RNA helicase DDX21 plays vital roles in ribosomal RNA biogenesis, transcription, and the regulation of host innate immunity during virus infection. DDX21 is composed of three domains, including the N‐terminal domain, the middle D1 and D2 domain, and the C‐terminal foldase domain. In summary, here we reported multiple sets of crystal structures of RNA helicase DDX21 either in ligand‐free (DDX21‐apo) or in complex with AMP (DDX21‐AMP), ADP (DDX21‐ADP), or a nonhydrolyzable ATP analog (AMPPNP) and a 15‐nucleotide poly(U) ssRNA (DDX21‐AMPPNP‐U15), corresponding to different unwinding states (except for DDX21‐AMP). We elucidated the conformational rearrangements upon the ATP and ssRNA binding during the dsRNA unwinding cycle, and described an RNA unwinding machinery including one wedge helix, one sensor motif V, and the DEVD box.

Therefore, we deleted the linker loop partially (GKKTQ; residue 401‐405) and generated a new construct (named as a del‐loop mutant), which helped us obtain a 1.8 Å resolution crystal structure of DDX21‐ADP and another DDX21‐apo structure with 3.1 Å resolution. Here, we have shown that the DDX21 helicase core adopted an open conformation in its apo‐state, and the success of crystallization either without the linker loop or del‐loop constructs indicated the vast flexibility of the open conformation in solution. When DDX21 was in the apo‐state, the RNA binding pocket was closed tightly. Three motifs in the D1 domain sterically clashed with the modeled ssRNA molecule, including residue Gly295 from motif Ib, residue Asp321 from motif Ic, and more significantly, residues Met347 and Phe349 adjacent to Gln352 which interacted with U4 in the RNA bound structure. A short loop (TGTG, named as “TG loop”) within the motif I had severe steric hindrance with the modeled AMPPNP in DDX21 apo‐structure; thus the ATP‐binding pocket was in the closed conformation. Comparison of the structures of DDX21 involved in the unwinding cycle revealed that the two conserved domains (D1 and D2) of helicase core unambiguously showed an “open” to “closed” conformational change between the apo‐state and post‐unwound state. From the apo‐ to post‐unwound state, D2 domain not only shifted ≈29 Å but also rotated by ≈180°; from the post‐unwound to post‐hydrolysis state, D2 shifted ≈24 Å and rotated by ≈100°; and from the post‐hydrolysis back to the apo‐state, D2 shifted ≈25 Å and rotated by ≈78°. First, the apo‐D1D2 core bound dsRNA in an ATP independent manner.

> SFSNFPISEETIKLLKGRGVTFLFPIQAKTFHHVYSGKDLIAQARTGTGKTFSFAIPLIEKLHGELQDRKRGRAPQVLVLAPTRELANQVSKDFSDITKKLSVACFYGGTPYGGQFERMRNGIDILVGTPGRIKDHIQNGKLDLTKLKHVVLDEVDQMLDMGFADQVEEILSVAYKKDSEDNPQTLLFSATCPHWVFNVAKKYMKSTYEQVDLIKTAITVEHLAIKCHWTQRAAVIGDVIRVYSGHQGRTIIFCETKKEAQELSQNSAIKQDAQSLHGDIPQKQREITLKGFRNGSFGVLVATNVAARGLDIPEVDLVIQSSPPKDVESYIHRSGRTGRAGRTGVCICFYQHKEEYQLVQVEQKAGIKFKRI>[2x]QVQQEPSAETSEGTGINITCSHPSIQAYSIQWYRQLPGRGPAFLVSAVKGSKEVPDPEGRLSVSADSRSSALWLARPRLGDAAVYYCAVRGSSYTKLTFGTGTRLSVQPHITPSPSVYRLTSEDNKNLEMCLITDYSPEKLDLSSVDSKTETVVEVATSENKHEASYLSTYWAKKDEMQCG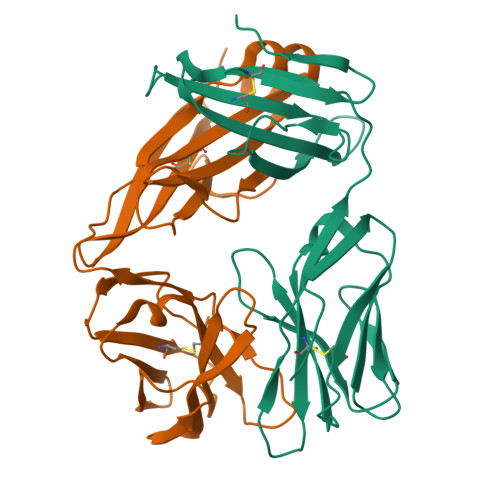AKHEGFGILKGDDPEAGASTVCITGMSLLFKTDENLN;>EINQPSILVLKEDENATLSCRQNDNHDYMSWYLQQPGKGLQLIYSSYGVKQENKGDIHTGYEAKRSSQEVFHLDIISAKKNHSAIYFCASSSYKGNTPLNFGQGTRLTVLGKNSEIIEPDVVIFSPSKQEIQEKKKATLVCLASGFFPDHLNLVWKVNGVKRTEGVGTDEISTSNGSTYSLTSRLRISAQEWFNPLNRFECIANFFKNGTQQSIQKIIYGDTGCDIFKENYQRSATAGK[2x]>MHHHHHHLILAPMVRVGTLPMRLLALDYGADIVYCEELIDLKMIQCKRVVNEVLSTVDFVAPDDRVVFRTCEREQNRVVFQMGTSDAERALAVARLVENDVAGIDVNMGCPKQYSTKGGMGAALLSDPDKIEKILSTLVKGTRRPVTCKIRILPSLEDTLSLVKRIERTGIAAIAVHGRKREERPQHPVSCEVIKAIADTLSIPVIANGGSHDHIQQYSDIEDF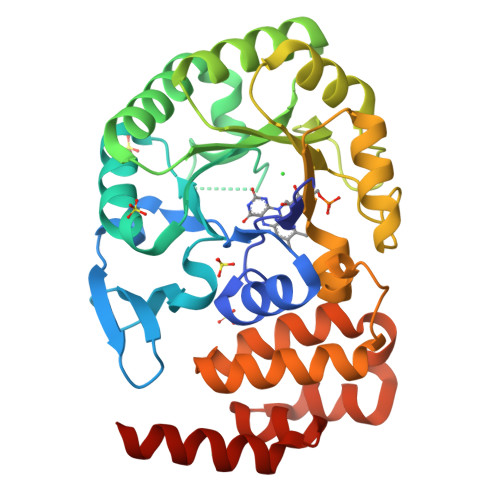RQATAASSVMVARAAMWNPSIFLKEGLRPLEEVMQKYIRYAVQYDNHYTNTKYCLCQMLREQLKSPQGRLLHAAQSSREICEAFGLGAFYEETTQELDAQQAR[2x]>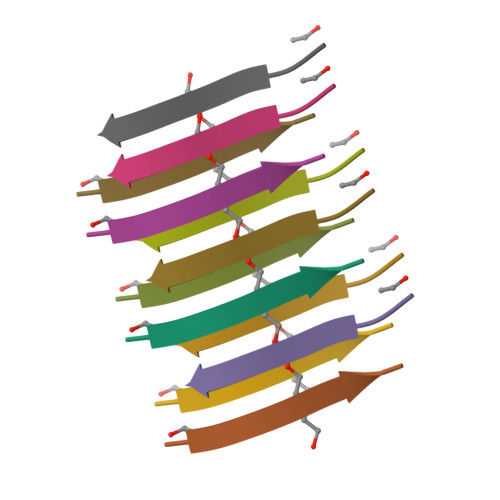SGMGGIT[2x]> GPIPTAPRENSLMFLSTTPDDTVPAYGNVRTPPVNYLPGEITDLLQLARIPTLMAFGRVPEPEPASDAYVPYVAVPTQFDDKPLISFPITLSDPVYQNTLVGAISSNFANYRGCIQITLTFCGPMMARGKFLLSYSPPNGTQPQTLSEAMQCTYSIWDIGLNSSWTFVIPYISPSDYRE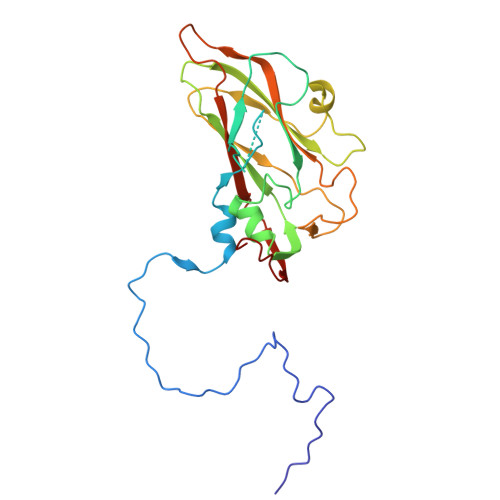TRAITNSVYSADGWFSLHKLTKITLPPDCPQSPCILFFASAGEDYTLRLPVDCNPSYVFH>[4x]SMLYQAALKEIPECIVYSKRFIVPDFSSYIKLIPPIGQEVMKANPGLTL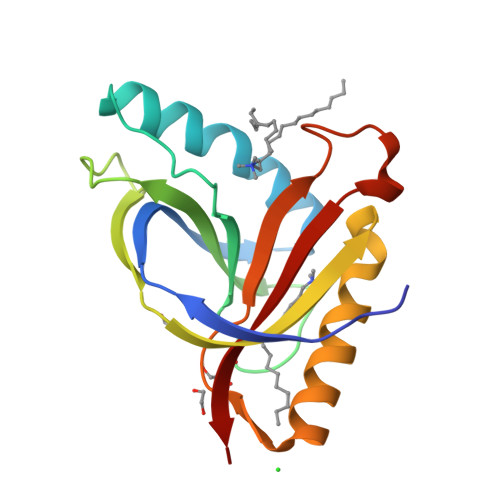TTPAYCFTLYHDKEYKEKNMDVEFCEAVNDFGKNEGNIIFQVIPAITAVTVIHKGPYDSLRNAYIYLMQWVEDNGYLLTNSPRESYIDGIWNKQDSAEWMTEIQFPVEKV>MKAVVQRVTRASVTVGGEQISAIGRGICVLLGISLEDTQKELEHMVRKILNLRVFEDESGKHWSKSVMDKQYEILCVSQFTLQCVLKGNKPDFHLAMPTEQAEGFYNSFLEQLRKTYRPELIKDGKFGAYMQVHIQNDGPVTIELESPAPGTATSDPKQLSKLEKQQQR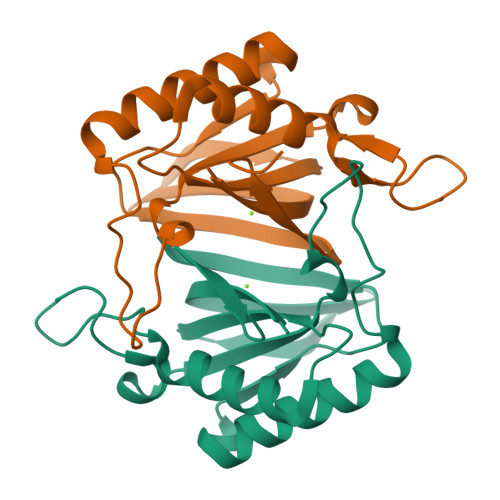KEKTRAKGPSESSKERNTPRKEDRSASSGAEGDVSSEREP[4x]> MGLPWELARFSIVKDEVLPHFATNEDLDLANEIISLFKAGKKLGEIDEEIEYLEKIYDHKLVRAFVKLLTRLCEFELDSPIPPIQIRRELFKYGPVLDEKEREDIIQKVSKKLGADIMRFVFSDLDEEKKIIKAPTISAEDLIRWYNLSLLQTLLFKA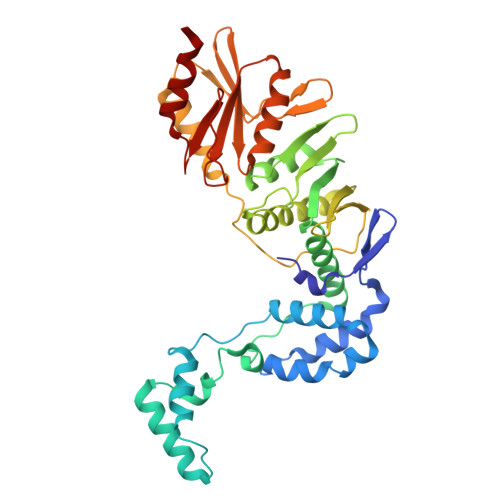YKLTVYVSSNWKEIIRRAKWLGLMYFAYDKPLRFEFLGPATLVKLTEKYGRNLAVLLQFIISSQNWKIEAELVLGKKFKRVYKLKLANFKELKELVIDEKRFDSSVEEKFYKDFTNVIKGWKIIREPEPLVVDNRVFIPDFLVEKGNLKVYVEIVGFWTKEYIKEKLDKLKKVKYPILILLNEELGKEKFNGMNVITYKRKIDISLVYKWLRELEN> GILYVIPAVYGVIILIGLIGNITLIKIFCTVKSMRNVPNLFISSLALGDLLLLITCAPVDASRYLADRWLFGRIGCKLIPFIQLTSVGVKVFTLTALSADRYKAIVRPMDIQASHALMKACLKAAFIWIISMLLAIPEAVFSDLHPFHEESTNQTFISCAPYPHSNELHPKIHSMASFLVF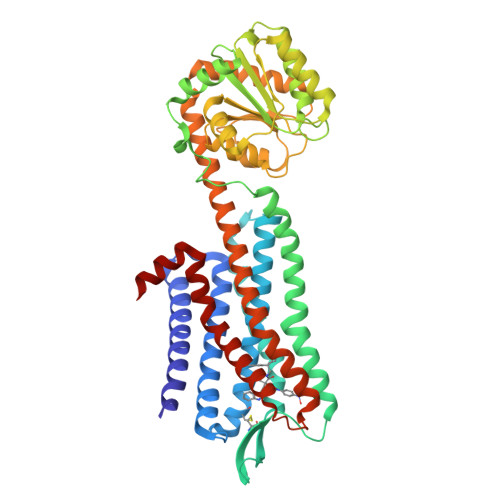YVIPLSIISVYYYFIAKNLIQSAGIDCSFWNESYLTGSRDERKKSLLSKFGMDEGVTFMFIGRFDRGQKGVDVLLKAIEILSSKKEFQEMRFIIIGKGDPELEGWARSLEEKHGNVKVITEMLSREFVRELYGSVDFVIIPSYFEPFGLVALEAMCLGAIPIASAVGGLRDIITNETGILVKAGDPGELANAILKALELSRSDLSKFRENCKKRAMSFSKQIESEKRLAKTVLVFVGLFAFCWLPNHVIYLYRSYHYSEVDTSMLHFVTSICARLLAFTNSCVNPFALYLLSKSFRKQFNTQL> MASMSNGTPDIIVNAQINSEDENVLDFIIEDEYYLKKRGVGAHIIKVASSPQLRLLYKN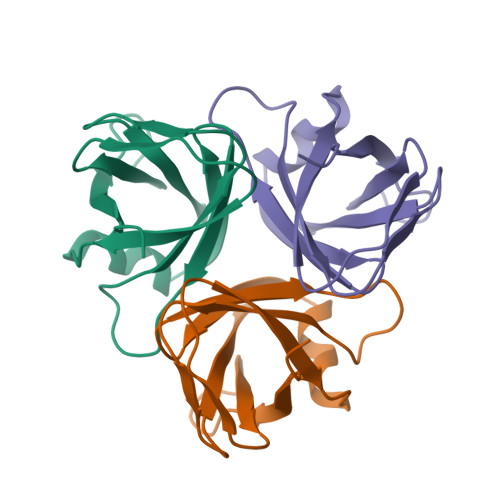AYSTVSCGNYGVLCNLVQNGEYDLNAIMFNCAEIKLNKGQMLFQTKIWR> MACAAARSPADQDRFICIYPAYLNNKKTIAEGRRIPISKAVENPTATEIQDVCSAVGLNVFLEKNKMYSREWNRDVQYRGRVRVQLKQEDGSLCLVQFPSR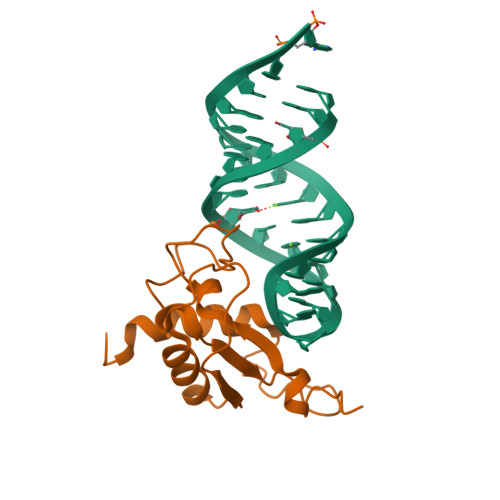KSVMLYAAEMIPKLKTRTQLEHHHHHH> GGGRNFTVLRKLNLVPIKKSVSSPKVCKPSPVKERVDHVFYQKFKSMALQELGTNYLSISYVPSLSKFLSKNLRSMKNCIVFFDKVEHIHQYAGIDRAVSETLSLVDINVVIIEMNDYLMKEGIQSS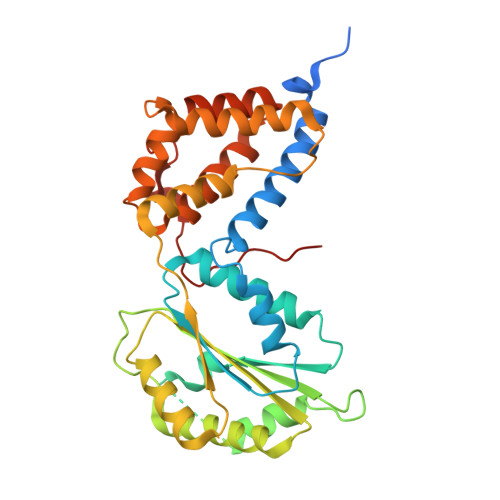KSKECIESMGQASYSGQLDFEASEKPSNHTSDLMMMVMRKINNDESIDHIVYFKFEQLDKLSTSTIIEPSKLTEFINVLSVLEKSNNIAFKVLIYSNNVSISSLLSTSLKKKLNTKYTVFEMPILTCAQEQEYLKKMIKFTFDSGSKLLQSYNSLVTCQLNNKESNLAIFFEFLKVFPHPFTYLFNAYTEIIVQSRTFDELLDKIRNRLTIKNYPHSAYNFKKNQRLPLKLTRKVHDR> ESA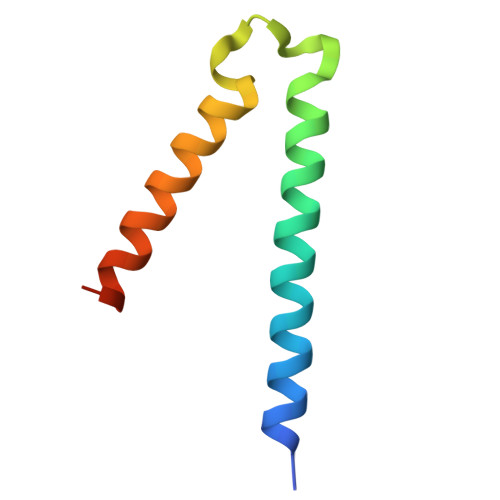FNQTEFNKLLLECVVKTQSSVAKILGIESLSPHVSGNSKFEYANMVEDIREKVSSEMERFFPKNDDE>MDVVSLDKPFMYFEEIDNELDYEPESANEVAKKLPYQGQLKLLLGELFFLSKLQRHGILDGATVVYIGSAPGTHIRYLRDHFYNLGVIIKWMLIDGRHHDPILNGLRDVTLVTRFVDEEYLRSIKKQLHPSKIILISDVASAAGGNEPSTADLLSNYALQNVMISILNPVASSLKWRCPFPDQWIKDFYIPHGNKMLQPFAPSYSAEMRLLSIYTGENMRLTRVTKSDAVNYEKKMYYLNKIVRNKVVVNFDYPNQEYDYFHMYFMLRTVYCNKTFPTTKAKVLFLQQSIFRFLNIP[2x];>[2x]MNRNPDQNTLPNITLKIIETYLGRVPSVNEYHMLKSQARNIQKITVFNKDIFVSLVKKNKKRFFSDVNTSASEIKDRILSYFSKQTQTYNIGKLFTIIELQSVLVTTYTDILGVLTIKAPNVISSKISYNVTSMEELARDMLNSMNVAVIDKAKVMGRHNVSSLVKNVNKLMEEYLRRHNKSCICYGSYSLYLINPNIRYGDIDILQTNSRTFLIDLAFLIKFITGNNIILSKIPYLRNYMVIKDENDNHIIDSFNIRQDTMNVVPKIFIDNIYIVDPTFQLLNMIKMFSQIDRLEDLSKDPEKFNARMATMLEYVRYTHGIVFDGKRNNMPMKCIIDENNRIVTVTTKDYFSFKKCLVYLDENVLSSDI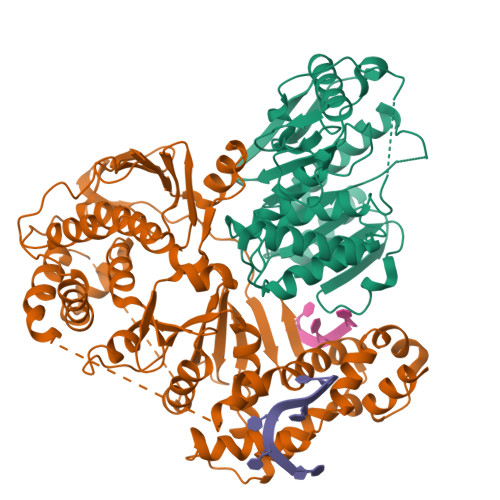LDLNADTSCDFESVTNSVYLIHDNIMYTYFSNTILLSDKGKVHEISARGLCAHILLYQMLTSGEYKQCLSDLLNSMMNRDKIPIYSHTERDKKPGRHGFINIEKDIIVF The mammalian SLC13 proteins are members of the larger divalent-anion sodium symporter (DASS) family. DASS proteins typically have a molecular weight of 45–65 kDa and form obligate homodimers. Each protomer consists of a scaffold and a transport domain. Structural information, along with cross-linking and computer modeling, indicates that DASS proteins operate in an elevator-type transport mechanism (Reyes et al., 2009; Drew and Boudker, 2016; Garaeva and Slotboom, 2020).

To obtain the structure of a DASS protein in a substrate-free, Na+-bound state, we purified VcINDY in 100 mM Na+, but in the absence of a substrate, for single-particle cryo-electron microscopy (cryo-EM). In a parallel approach, we used amphipol polymer to preserve the transporter protein, which allowed data collection on particularly thin ice to maximize signal-to-noise. This VcINDY structure in amphipol, without Fab, was determined to 3.16 Å resolution. The two cryo-EM structures of VcINDY are in a substrate-free, inward-facing (Ci-Na+) state and provide an opportunity to describe the conformational changes that occur upon substrate release. The Ci-Na+ VcINDY structures are very similar to each other, with an r.m.s.d of 0.75 Å. Comparison of the previous Ci-Na+-S and amphipol preserved Ci-Na+ VcINDY structures also revealed prominent changes on the periplasmic surface. The loop connecting HPoutb and TM10a, from Ala395 to Pro400, has moved on the periplasmic surface. The C-terminus of HPoutb also unwinds by one turn (Val392 – Glu394) in the amphipol structure. As a result, the conserved salt bridge between Glu394 with Lys337 of H9b from the scaffold domain breaks, and Phe396 moves away from its contact with H9c. Finally, the side chain of Trp461 is inserted between TM6, TM10a and TM11, packing against another conserved aromatic residue, Phe220.

>[2x]REWFLHRNSLIVLADVALFLALYHFLPFEHNVVLGISMLAFIAVLWLTEALHVTVTAILVPVMAVFFGIFETQAALNNFANSIIFLFLGGFALAAAMHHQGLDKVIADKVLAMAQGKMSVAVFMLFGVTALLSMWISNTATAAMMLPLVLGVLSKVDADKQRSTYVFVLLGVAYSASIGGIATLVGSPPNAIAAAEVGLSFTDWMKFGLPTAMMMLPMAIAILYFLLKPTLNGMFELDRAPVNWDKGKVVTLGIFGLTVFLWIFSSPINAALGGFKSFDTLVALGAILMLSFARVVHWKEIQKTADWGVLLLFGGGLCLSNVLKQTGTSVFLANALSDMVSHMGIFVVILVVATFVVFLTEFASNTASAALLIPVFATVAEAFGMSPVLLSVLIAVAASCAFMLPVATPPNAIVFASGHIKQSEMMRVGLYLNIACIGLLTAIAMLFWQ> AECSSELYTEASGYISSLEYPRSYPPDLRCNYSIRVERGLTLHLK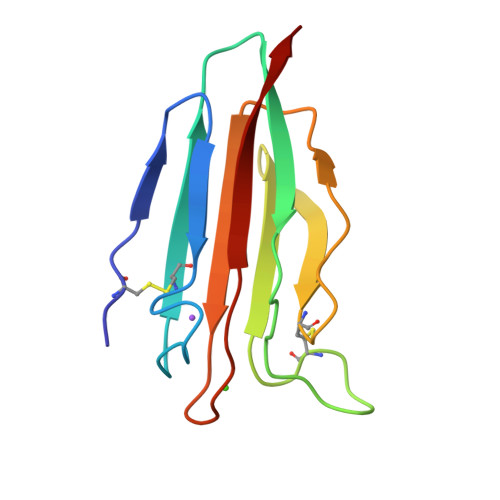FLEPFDIEDHPEVPCPYDQLQIYANGKNIGEFCGKQRPPDLDTSSNAVDLLFFTDESGDSRGWKLRYTTEII> AAGCGCCUGGACUUAAAGCCAUUGCACU;> CCGGCUUUAAGUUGACGAGGGCAGGGUUUAUCGAGACAUCGGCGGGUGCC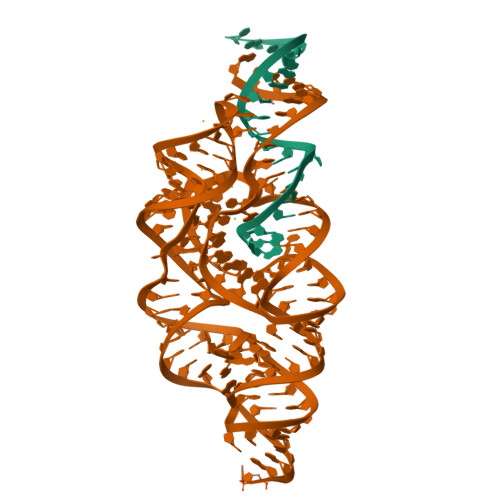CUGCGGUCUUCCUGCGACCGUUAGAGGACUGGUAAAACCACAGGCGACUGUGGCAUAGAGCAGUCCGGGCAGGAA>GAMAKVQVNNVVVLDNPSPFYNPFQFEITFECIEDLSEDL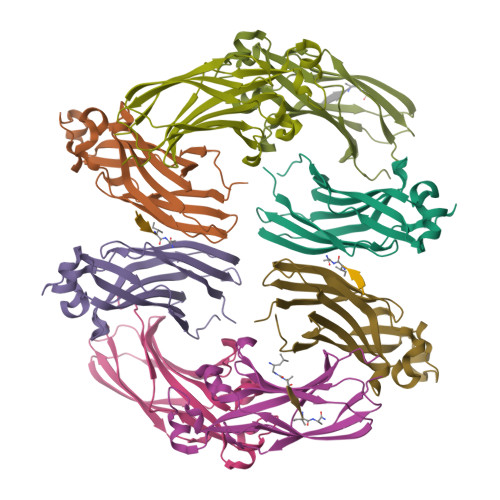EWKIIYVGSAESEEYDQVLDSVLVGPVPAGRHMFVFQADAPNPGLIPDADAVGVTVVLITCTYRGQEFIRVGYYVNNEYTETELRENPPVKPDFSKLQRNILASNPRVTRFHINWEDN[8x]> TETQPPVTNLSVSVENLCTVIWTWNPPEGASSNCSLWYFSHFGDKQDKKIAPETRRSIEVPLNERICLQVGSQCSTNESEKPSILVEKCISPPEGDPESAVTELQCIWHNLSYMKCSWLPGRNTSPDTNYTLYYWHRSLEKIHQCENIFREGQYFGCSFDLTKVKDSSFEQHSVQIMVKDNAGKIKPSFNIVPLTSRVKPDPP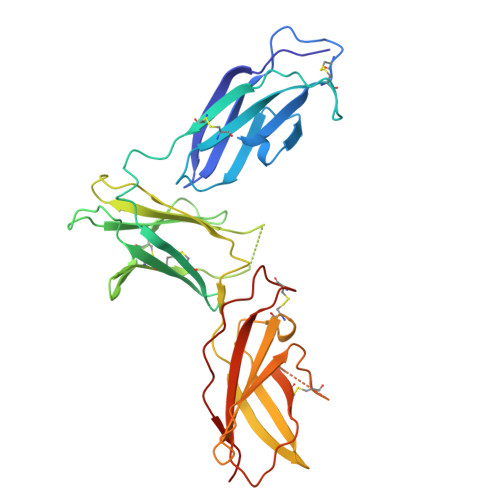HIKNLSFHNDDLYVQWENPQNFISRCLFYEVEVNNSQTETHNVFYVQEAKCENPEFERNVENTSCFMVPGVLPDTLNTVRIRVKTNKLCYEDDKLWSNWSQEMSIGKKRNS>EAEFGKCGPPPPIDNGDITSFPLSVYAPASSVEYQCQNLYQLEGNKRITCRNGQWSEPPKC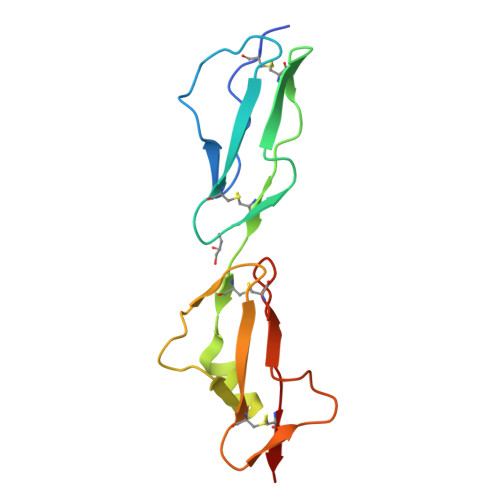LHPCVISREIMENYNIALRWRAKQKLYSRTGESVEFVCKRGYRLSSRSHTLRTTCWDGKLEYPTCAKR[2x]>GAGPLDLLSREELLTDTSNSSSSTGEEGDLAALLPDLSGRLLINSVFHMGAERLQQMLFSDSPFLQGFLQQRKFTDVTLSPWSSDSKCHQRRVLTYTIPISNQLGPKSASVVETQTLFRRGPQAGGCVVDSEVLTQGIPYQDYFYTAHRYCILG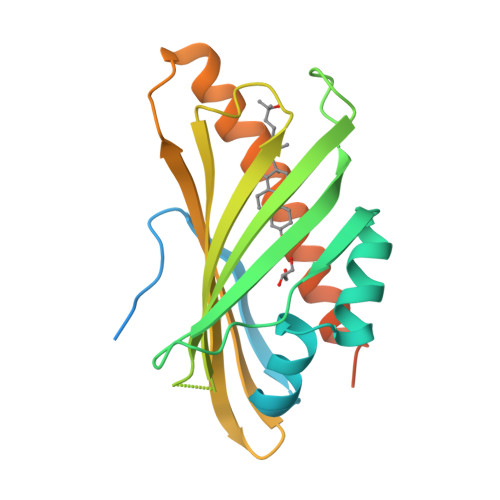LARNKARLRVSSEIRYRKQPWSLVKSLIEKNSWSGIEDYFHHLDRELAKAEKLSLEEGGKDTRGLLSGLRRRKRPLS[4x]>[2x]MDLSGKMVKQVEILSDGIVFYEIFRYRLYLISEMSPVNIQGVDLLEGNWGTVGSVIFFKYTIDGKEKTAKDIVEAIDEETKSVTFKIVEGDLMELYKTFIII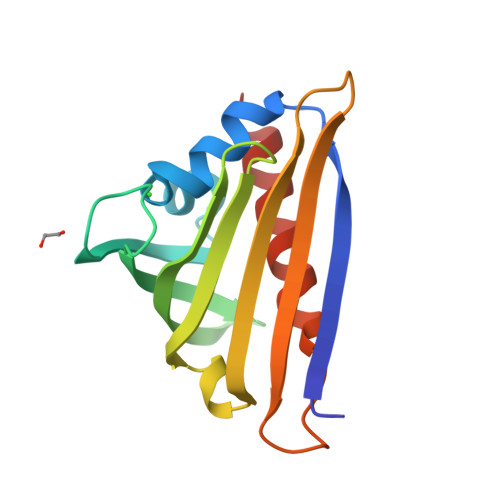VQVDTKGEHNSVTWTFHYEKLKEDVEEPNTLMNFCIEITKDIETYHLK(3R,4R)-1-METHANESULFONYL-PYRROLIDINE-3,4-DICARBOXYLIC ACID 3-[(4-CHLORO-PHENYL)-AMIDE] 4-{[2-FLUORO-4-(2-OXO-2H-PYRIDIN-1-YL)-PHENYL]-AMIDE} | C24 H22 Cl F N4 O5 S | 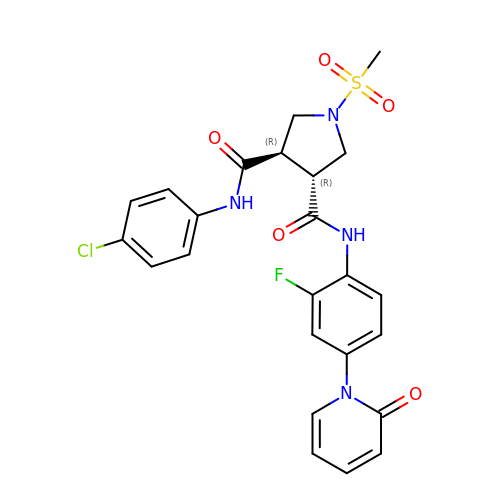CUZHVTKMXOGVKA-OALUTQOASA-N>[2x]MSLTQHLVITAVGTDRPGICNEVVRLVTQAGCNIIDSRIAMFGKEFTLLMLI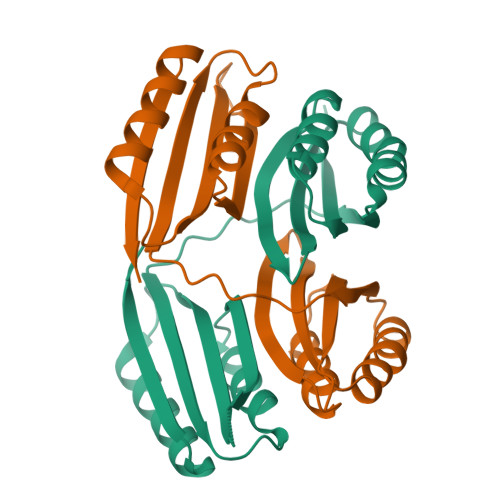SGSPSNITRVETTLPLLGQQHDLITMMKRTSPHDHQTHAYTVEVYVESDDKLGLTEKFTQFFAQRQIGMASLSAQTISKDKLHSEQNQFHIAISARVDSGCNLMQLQEEFDALCTALDVQGSLNFIKNSQEGGSHHHHHH> GRNDGEGLGGTFQKIPVALLTTTGRKTGQPRVNPLYFLRDGGRVIVAASKGGAEKNPMWYLNLKANPKVQVQIKKEVLDLTARDATDEERAEYWPQLVTMYPSYQDYQSWTDRTIPI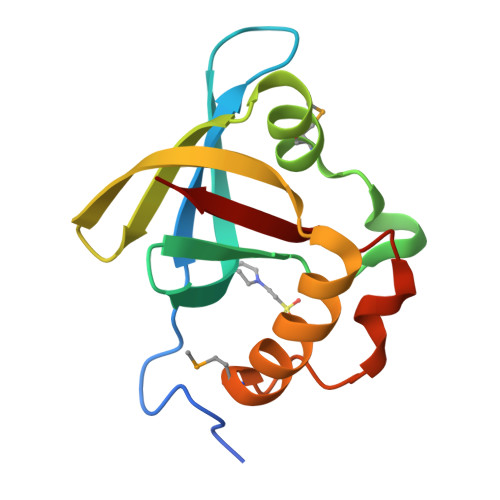VVCEP> SRSTHNEMEKNRRAHLRLSLEKLKGLVPLGPDSSRHTTLSLLTKAKLHIKKLEDSDRKAVHQIDQLQRE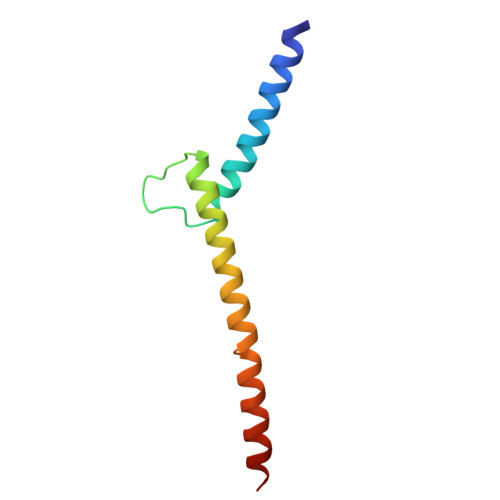QRHLKRQLEKL(1~{S})-~{N}'-(4-azanylbutyl)-~{N}"-(2-methoxyethyl)methanetriamine 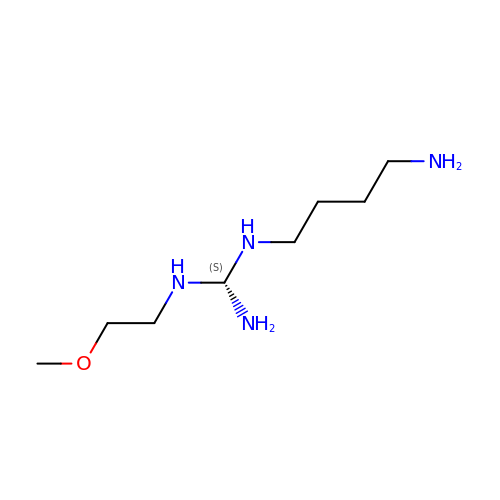| C8 H22 N4 O | HBYRDDGQNQMGCZ-QMMMGPOBSA-N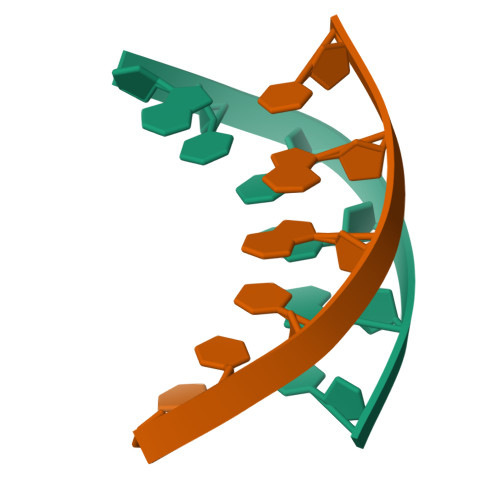>ATTAAT[5x]> MAKFEDKVDLYDDRGNLVEEQVPLEALSPLRNPAIKSIVQGIKRTVAVNLEGIENALKTAKVGGPACKIMGRELDLDIVGNAESIAAAAKEMIQVTEDDDTNVELLGGGKRALVQVPSARFDVAAEYSAAPLVTATAFVQAIINEFDVSMYDANMVKAAVLGRYPQSVEYMGANIATMLDIPQKLEGPGYALRNIMVNHVVAATLKNTLQAAALSTILEQTAMFEMGDAVGAFERMHLLGLAYQGMNADNLVFDLVKANGKEGTVGSVIA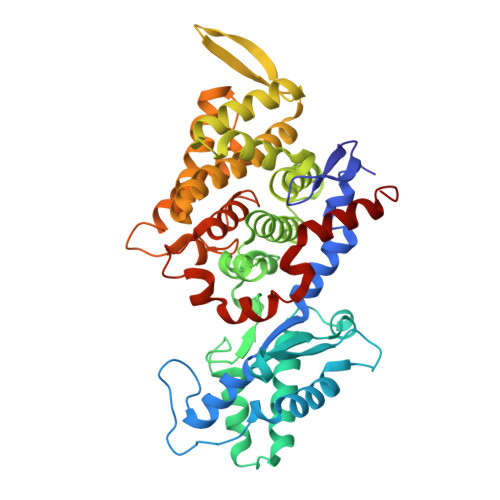DLVERALEDGVIKVEKELTDYKVYGTDDLAMWNAYAAAGLMAATMVNQGAARAAQGVSSTLLYYNDLIEFETGLPSVDFGKVEGTAVGFSFFSHSIYGGGGPGIFNGNHIVTRHSKGFAIPCVAAAMALDAGTQMFSPEATSGLIKEVFSQVDEFREPLKYVVEAAAEIKNEI> 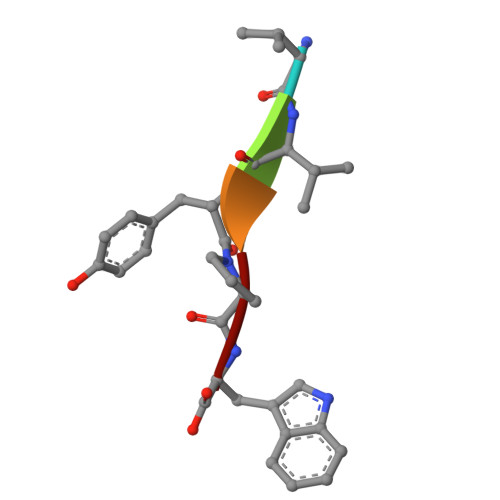VVYPW>SDIAFLIDGSGSIIPHDFRRMKEFVSTVMEQLKKSKTLFSLMQYSEEFRIHFTFKEFQNNPNPRSLVKPITQLLGRTHTATGIRKVVRELFNITNGARKNAFKILVVI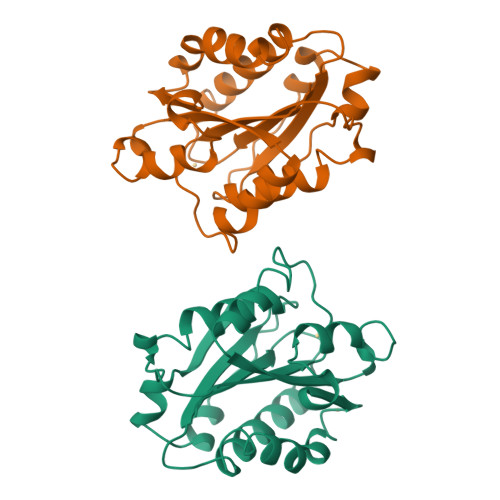TDGEKFGDPLGYEDVIPEADREGVIRYVIGVGDAFRSEKSRQELNTIASKPPRDHVFQVNNFEALKTIQNQLREKIFAIEG[2x]> DTPFIRPDMKAFLEAIAAMAGPTLAEMTLEEARASYVALHGMADRPARELAVIRNLSCPGPAGDIPLRLYDARESREAGPVITFYHGGGFVIGDLDTHHNLCTEIAALMDLPVVAVDYRLAPEH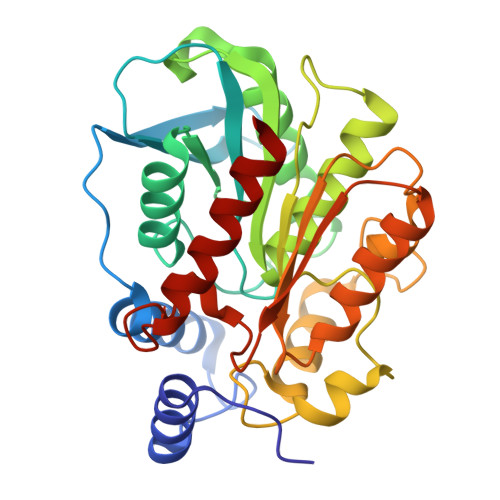PFPAAIEDCEAATRWVASSPSELGRTASGVIPIGDAAGGNATIVVSQLLGAKPADVPVVLQVPIFPLASDAVGSASLEAFAEGFVLTKASIEFFDTAYKADRADPRGFPILGDHTAAPPTIVATASLDPIRDSGRDYAKALVEAGRDVVYLEMEGVTHSFTNIRAAVPSTQGDLERIIAAMKMMLG>[2x]MENQLTKSVEERTFQYQDSLPSLPVPALEESLKKYLESVKPFANEDEYKKTEEIVQKF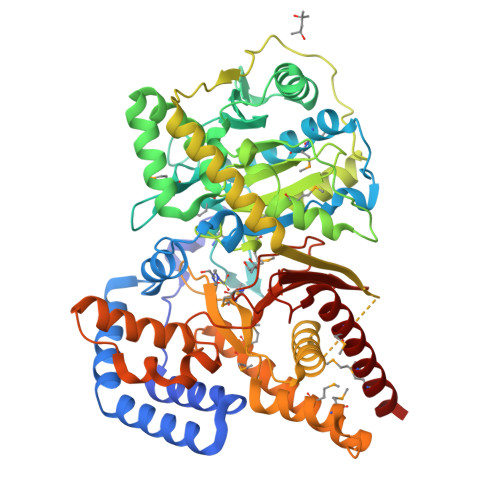QEGAGKRLHQKLLERARGKRNWLEEWWLNVAYLDVRIPSQLNVNFVGPCPHFEHYWPAREGTQLERGSMMLWHNLNYWQLLRREKLPVHKSGNTPLDMNQFRMLFSTCKVPGITRDSIMNYFKTESEGHCPTHIAVLCRGRAFVFDVLHEGCLITPPELLRQLTYIHKKCSNEPVGPSIAALTSEERTRWAKAREYLISLDPENLTLLEKIQTSLFVYSIEDSSPHATPEEYSQVFEMLLGGDPSVRWGDKSYNLISFANGIFGCCCDHAPYDAMVMVNIAHYVDERVLETEGRWKGSEKVRDIPLPEELVFTVDEKILNDVSQAKAQHLKAASDLQIAASTFTSFGKKLTKEEALHPDTFIQLALQLAYYRLHGRPGCCYETAMTRYFYHGRTETVRSCTVEAVRWCQSMQDPSASLLERQQKMLEAFAKHNKMMKDCSHGKGFDRHLLGLLLIAKEEGLPVPELFEDPLFSRSGGGGNFVLSTSLVGYLRVQGVVVPMVHNGYGFFYHIRDDRFVVACSSWRSCPETDAEKLVQMIFHAFHDMIQLMNTAHL>MIIERLVGNLRDLNPLDFSVDYVDLEWFETRKKIARFKTRQGKDIAIRLKDAPKLGLSQGDILFKEEKEIIAVNILDSEVIHIQAKSVAEVAKICYEIGNRHAALYYGESQFEFKTPFEKPTLALLEKLGVQ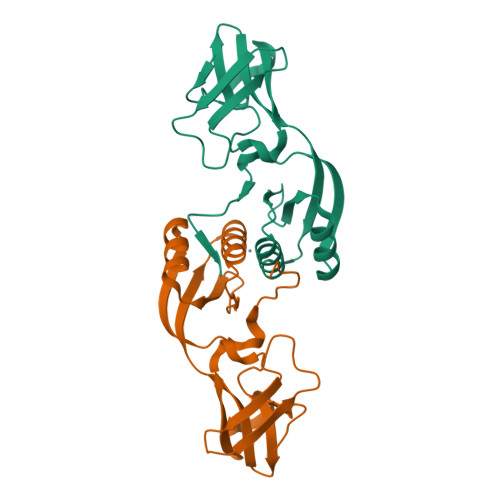NRVLSSKLDSKERLTVSMPHSEPNFKVSLASDFKVVVK[4x]>MDYTIENNMIKVVISDHGAEIQSVKSAHTDEEFMWQANPEIWGRHAPVLFPIVGRLKNDEYTYKGKTYHLGQHGFARNADFEVENHTKESITFLLKDNEETRKVYPFKFEFRVNYNLMNNLLEENFSVVNKSDETMIFGVGGHPGFNLPTDHGENKEDFYFDMHPSVTRVRIPLKDASLDWNNRSLAPTDSLIALSDDLFKDDALIYELRGNDNKVSLRTDKNKFHVNVW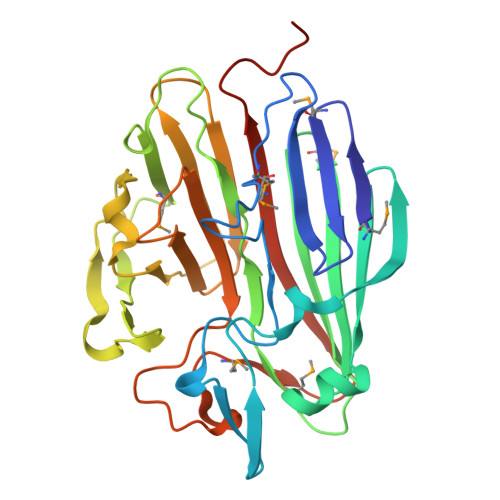TRDAPFVGIWSQYPKTDNYVCIEPWWGIADRDDADGDLEHKYGMNHLKPGKEFQAGFSMTYHSTTDEVKLEHHHHHH[2x]>[2x]GSMAQILPIRFQEHLQLQNLGINPANIGFSTLTMESDKFICIREKVGEQAQVVIIDMNDPSNPIRRPISADSAIMNPASKVIALKAGKTLQIFNIEMKSKMKAHTMTDDVTFWKWISLNTVALVTDNAVYHWSMEGESQPVKMFDRHSSLAGCQIINYRTDAKQKWLLLTGISAQQNRVVGAMQLYSVDRKVSQPIEGHAASFAQFKMEGNAEESTLFCF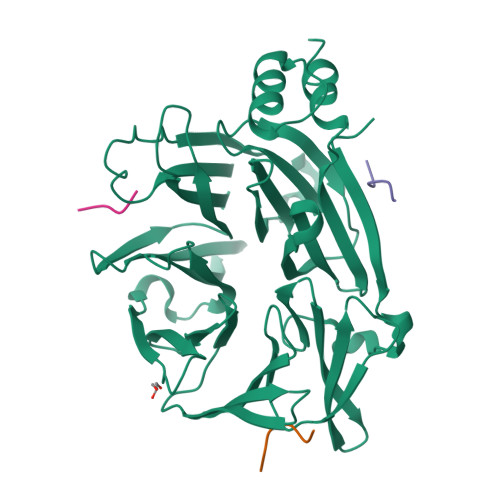AVRGQAGGKLHIIEVGTPPTGNQPFPKKAVDVFFPPEAQNDFPVAMQISEKHDVVFLITKYGYIHLYDLETGTCIYMNRISGETIFVTAPHEATAGIIGVNRKGQVLSVCVEEENIIPYITNVLQNPDLALRMAVRNNLAGAEEL;>SPRLPLLES[6x]> GSYPWILNHDHSKQKEISDWLTFEIKDFVAYISPSREEIEIRNQTISTIREAVKQLWPDADLHVFGSYSTDLYLPGSDIDCVVTSELGGKESRNNLYSLASHLKKKNLATEVEVVAKARVPIIKFVEPHSGIHIAVSFERTNGIEAAKLIREWLDDTPGLRELVLIVKQFLHARRLNNVHTGGLGGFSIICLVFSFLHMHPRIITNEIDPKDNLGVLLIEFFELYGKNFGYDDVALGSSDGYPVYFPKSTWSAIQPIKNPFSLAIQDPGDESNNISRGSFNIRDIKKAFAGAFDLLTNRCFELHSATFKDRLGKSILGNVIKY;> GSWKKVQCTLCKSKKHSKERCPSIWRAYILVDDNEKAKPKVLPFHTIYCYNCGGKGHFG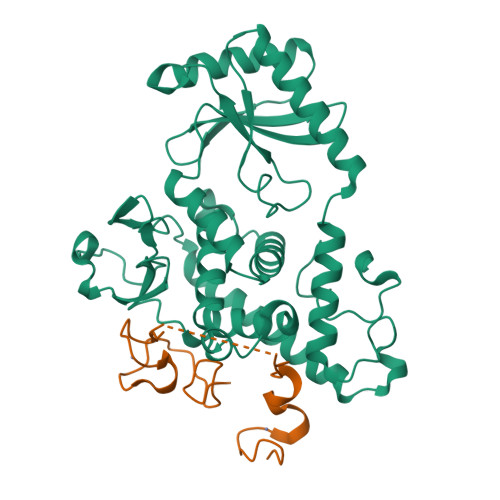DDCKEKRSSRVPNEDGSAFTGSNL>[8x]MAVELGVLLVRPRPGTGLGRVMRTLLLVLWLATRGSALYFHIGETEKKCFIEEIPDETMVIGNYRTQLYDKQREEYQPATPGLGMFVEVKDPEDKVILARQYGSEGRFTFTSHTPGEHQICLHSNSTKFSLFAGGMLRVHLDIQVGEHANDYAEIAAKDKLSELQLRVRQLVEQVEQIQKEQNYQRWREERFRQTSESTNQRVLWWSILQTLILVAIGVWQMRHLKSFFEAKKLV

TMED9 is a member of the TMED family of cargo receptors that facilitate the bidirectional transport of membrane proteins at the endoplasmic reticulum (ER)–Golgi interface via anterograde COPII and retrograde COPI vesicles. In addition, all TMEDs share a conserved domain architecture with luminal Golgi-dynamics (GOLD) and coiled-coil (CC) domains and a single TM domain. Sorting signals for COPI (dilysine motif, KK) and COPII (diphenylalanine motif, FF) coatomer proteins are contained in the cytosolic tail of TMED9. Here, we report cryo–electron microscopy (cryo-EM) structures of full-length TMED9 in octameric and dodecameric forms.

An unexpected feature of the TMED9 oligomers is an intrinsic symmetry mismatch between the CC and TM domains. In the homo-octamer, the TM domain consists of a dimer of tetramers, whereas the CC domain forms a dimer of trimers; for two of the eight subunits of the TMED9 octamer, the density of the CC domain was absent. Specifically, we noted that each TM tetramer has internal twofold symmetry, and twofold symmetry is also evident between the TM tetramers. In contrast to the symmetry of the TM domain, the CC domain formed obligate trimeric coiled coils, as was also predicted by MultiCoil. Within the TM domain interface, residues L214 and L225 constitute two layers of Leu-mediated hydrophobic interactions. Within the CC domain interface, four layers of Ile/Leu-mediated hydrophobic interactions are centered at residues L161, L164, L171, and I178. PIP (36:2) fits well with the cryo-EM density at both the headgroup and the acyl chains. The PIP headgroup between the TM tetramers is within hydrogen bonding distance to the R223 and H224 side chains from two of the four subunits at the tetramer-tetramer interface; these interactions could further stabilize octameric, dodecameric, or higher-order TMED9 complexes. The importance of the observed molecular interactions is supported by delayed elution from the gel filtration column for CC domain mutation E190R, the PIP-interacting residue mutation R223E and CC interface mutations Q177A, R191E, and W205A, all of which compromised TMED9 oligomerization. In addition, we used mass photometry, a label-free single-molecule technique for mass determination, and found that wild-type (WT) TMED9 has a mass distribution consistent with octamers and higher-order oligomers (such as dodecamers).> GMRADALKRREHIITTTCNLYRTHHHDSLTMENIAEQAGVGVATLYRNFPDRFTLDMACAQYLFNVVISLQLQAISTFPTDPEGVWTSFNQLLFDRGLGSLVPALAPESLDDLPDEVSALRRTTEKNTTTLINLAKQHGLVHHDIAPGTYIVGLITISRPPITALATISENSHKALLGLYLSGLKHGMMA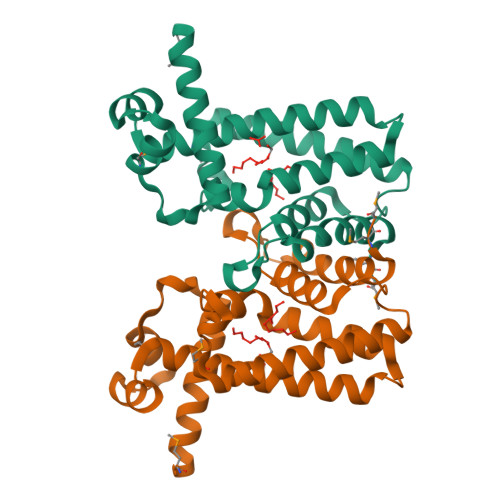NIGEHDGKS> NIGMILKERQDGVLVLTLNRPEKLNAITGELLDALYAALKEGEEDREVRALLLTGAGRAFSAGQDLTEFGDRKPDYEAHLRRYNRVVEALSGLEKPLVVAVNGVAAGAGMSLALWGDLRLAAVGASFTTAFVRIGLVPDSGLSFLLPRLVGLAKAQELLLLSPRLSAEEALALGLVHRVVPAEKLMEEALSLA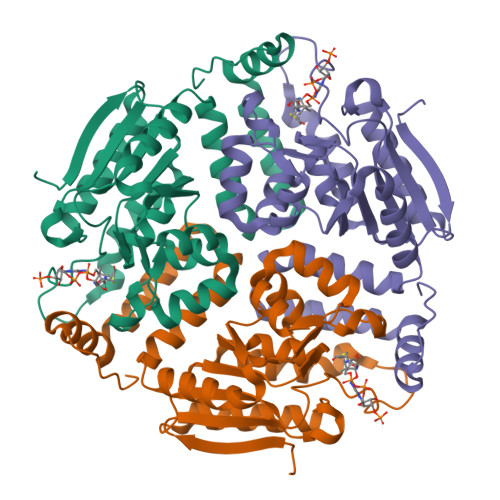KELAQGPTRAYALTKKLLLETYRLSLTEALALEAVLQGQAGQTQDHEEGVRAFREKRPPRFQGR>[2x]ERALLFTKPPSD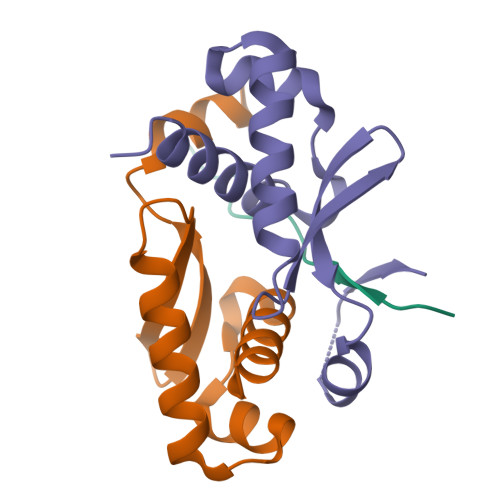LSAYAD;>[4x]GSHMGALKPAKAIVEALLFAAGDEGLSLSQIAAVLEVSELEAKAVIEELQQDCRREERGIQLVELGGVFLLATKKEHAPYLKKLVEAPGASP>[14x]MTDAELSPTDWVREQTERILEQGTTDGVHVLDRPIVLFTTTGAKSGKKRYVPLMRVEENGKYAMVASK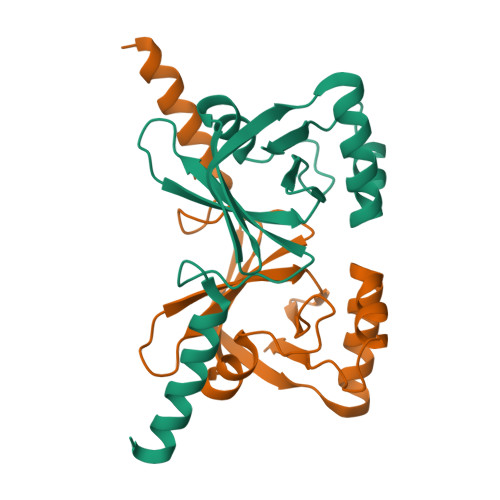GGDPKHPSWYFNVKANPTVSVQDGDKVLPDRTARELEGEEREHWWKLAVEAYPPYAEYQTKTDRLIPVFIVE>MLAGVKKDIEKLYEAVPQLSNVFKIEDKIGEGTFSSVYLATAQLQVGPEEKIALKHLIPTSHPIRIAAELQCLTVAGGQDNVMGVKYCFRKNDHVVIAMPYLEHESFLDILNSLSFQEVREYMLNLFKALKR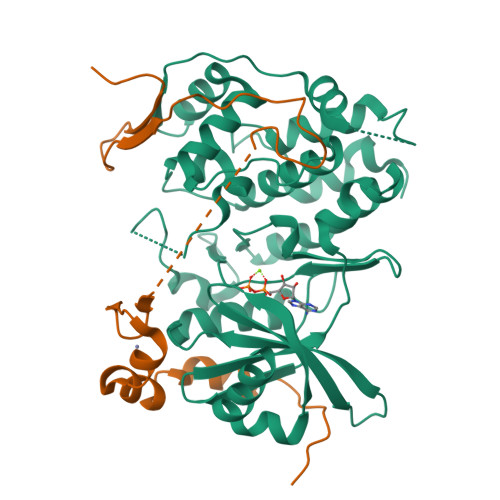IHQFGIVHRDVKPSNFLYNRRLKKYALVDFGLAQGTHDTKIELLKFVQSEAQQERCSQNKCSICLSRRQQVAPRAGTPGFRAPEVLTKCPNQTTAIDMWSAGVIFLSLLSGRYPFYKASDDLTALAQIMTIRGSRETIQAAKTFGKSILCSKEVPAQDLRKLCERLRGMDSSTPKLTSDIQGHATNLEGWNEVPDEAYDLLDKLLDLNPASRITAEEALLHPFFKDMSL[2x];>GPGTRTGRLKKPFVKVEDMSQLYRPFYLQLTNMPFINYSIQKPCSPFDVDKPSSMQKQTQVKLRIQTDGDKYGGTSIQLQLKEKKKKGYCECCLQKYEDLETHLLSEQHRNFAQSNQYQVVDDIVSKLVFDFVEYEKDTPKKKR[2x]1-(2,3,4-trihydroxyphenyl)nonan-1-one | C15 H22 O4 | 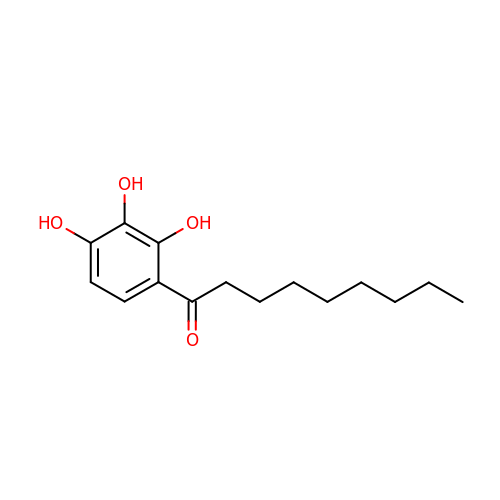ANXCQMITRFACCB-UHFFFAOYSA-N>[5x]MYMSKYVPVYTLLILIYSFNASAEWTGDKTNAYYSDEVISELHVGQIDTSPYFCIKTVKANGSGTPVVACAV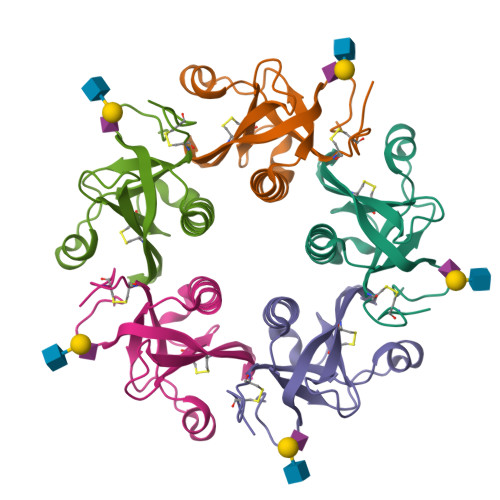SKQSIWAPSFKELLDQARYFYSTGQSVRIHVQKNIWTYPLFVNTFSANALVGLSSCSATQCFGPKLEHHHHHH> MWSSLFGWTSSNAKNKESPTKAIVRLREHINLLSKKQSHLRTQITNQENEARIFLTKGNKVMAKNALKKKKTIEQLLSKVEGTMESMEQQLFSIESANLNLETMRAMQEGAKAMKTIHSGLD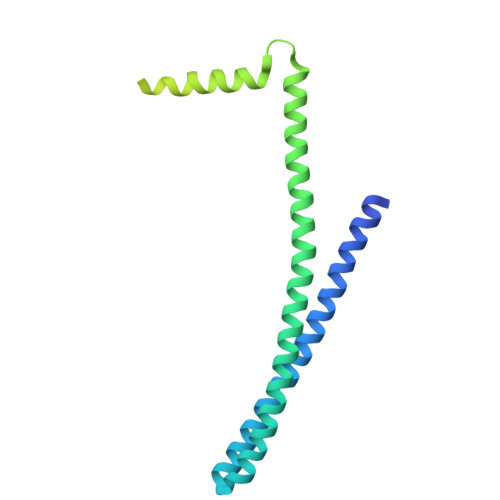IDKVDETMDEIREQVELGDEISDAISRPGGGGGGGGGGGGGGGLITGANEVDEDELDEELDMLAQENANQETSKIVNNNVNAAPISENKVSLPSVPSNKIKQSENSVKDGEEEEDEEDEDEKALRELQAEMGL> MHEGVHRKPSLLAHPGPLVKSEETVILQCWSDVMFEHFLLHREGMFNDTLRLIGEHHDGVSKANFSISRMTQDLAGTYRCYGSVTHSPYQVSAPSDPLDIVIIGLYEKPSLSAQPGPTVLAGENVTLSCSSRSSYDMYHLSRE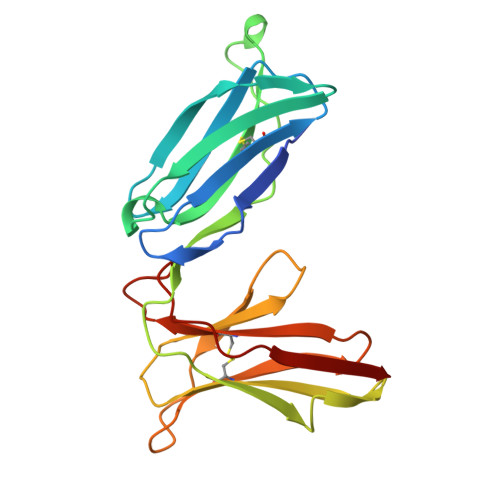GEAHERRLPAGPKVNGTFQADFPLGPATHGGTYRCFGSFHDSPYEWSKSSDPLLVSVT> MGSNPPASPLQDNLVIALHSYEPSHDGDLGFE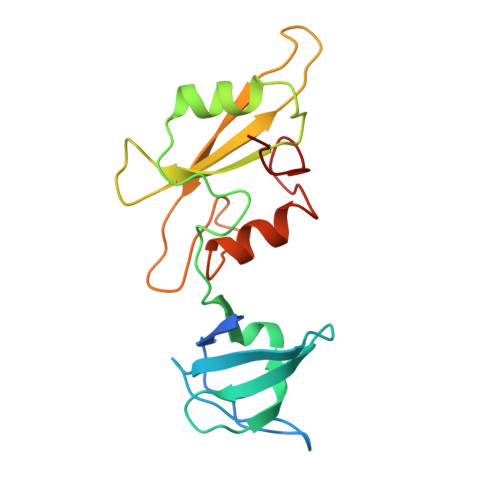KGEQLRILEQSGEWWKAQSLTTGQEGFIPFNFVAKANSLEPEPWFFKNLSRKDAERQLLAPGNTHGSFLIRESESTAGSFSLSVRDFDQNQGEVVKHYKIRNLDNGGFYISPRITFPGLHELVRHYTNASDGLCTRLSRPCQT6,7,8-trimethoxy-4-methylquinolin-2(1H)-one 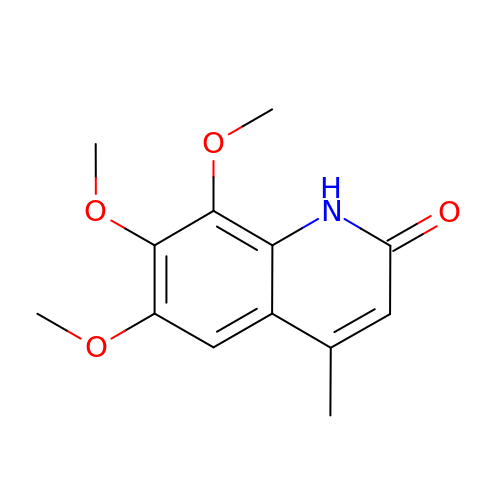| C13 H15 N O4 | JAKHLWMOJRMVRW-UHFFFAOYSA-N> MTSISHPVAPSQSTGNFDLFVVGSGFFGLTIAERAATQLGKRVLVIERRPHIGGNAYSEPEPETGIEVHKYGAHLFHTSNKRVWDYVRQFTDFTGYQHRVFAMHNGQAYQFPMGLGLVSQFFGRYFSPDEARALIAEQASEIDTKDAKNFEEKAISLVGRPLYEAFIKHYTAKQWQTDPKDLPASNITRLPVRYTFDNRYFNDTYEGLPVEGYTKWLENMAADERIEVRLDTDWFDVRDDLRAANPDAPVVYTGPLDRYFDYAEGRLGWRTLDFELEVLETGDFQGTPVMNYND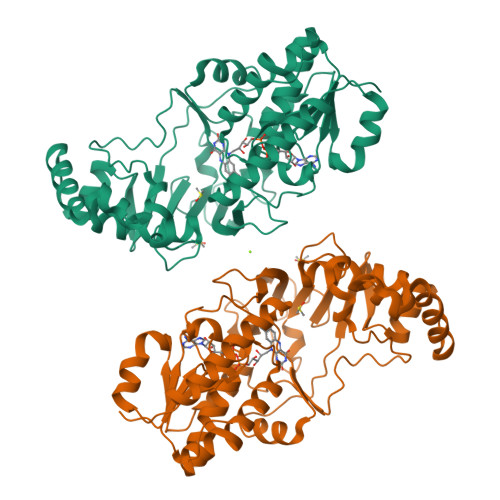LDVPYTRIHEFRHFHPERTYPTDKTVIMREYSRFADNDDEPYYPINTEADRAVLAAYRARAKAETASAKVLFGGRLGTYQYLDMHMAIASALSMFDNVLAPHLSEGASLVTEDESSKAHHHHHH>[2x]MSRKKNPSVIQFEKAITEKNYEAACTELLDILNKIDTNFGDIEGIDFDYPQQLETLMQDRIVYFCTRMSNAITQLFCDPQFSLSESGANRFFVVQRWLNLIFASSPYINADHILQTYNCNPERDSIYDIYLEPNKNVLMKFAVLYLPESNVNLNLDTMWETDKNICGSLCFALQSPRFIGTPAAFSKRSTILQWFPAKLEQFHVLDDLPSNISHDVYMHCSYDTAENKHNVKKALNQVIRSHLLKCGWQDRQITQIGMRNGKPVMVVVLEHFHSSHSIYRTHSTSMIAAREQFYLIGLGNNAVDQAGRDVFDEFHEFDGSNILKKLAFLKEMCEKNDAAVLYMPSIGMDLATIFVSNARFAPIQVIALGHPATTHSEFIEYVIVEDDYVGSESCFSETLLRLPKDALPYVPSSLAPTDVQYVLRETPEVVNIGIAATTMKLNPYFLETL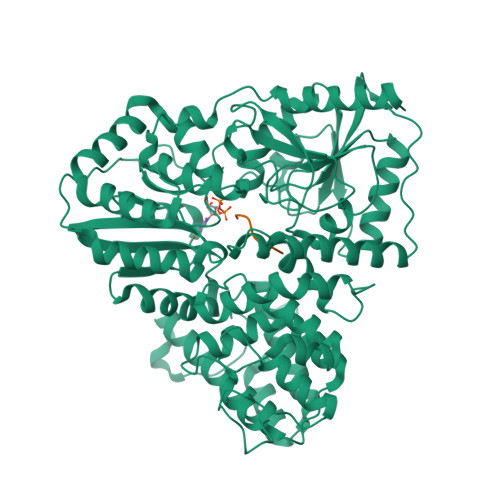KTIRDRAKVKVHFHFALGQSIGITHPYVARFIRSYLGDDATAHPHSPYNRYLDILHNCDMMLNPFPFGNTNGIIDMVTLGLVGVCKTGPEVHEHIDEGLFKRLGLPEWLIADSVEDYIERAIRLAENHQERLALRRHIIENNGLKTLFSGDPSPMGKTLFAKLTEWRQTNGI;>FGNWTT[2x]>[6x]MSDEPIIYINGDYLPLSQARVS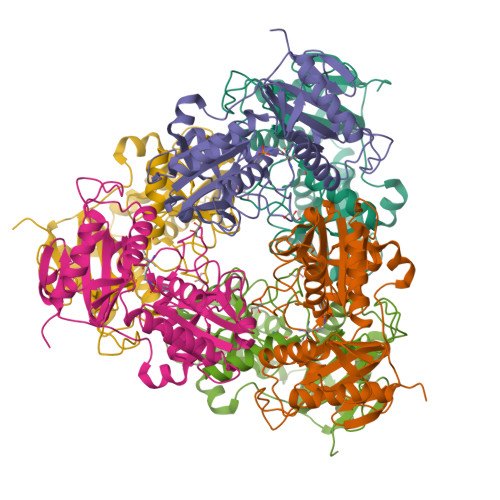PVDQGFLLGDGVFDVVSAWKGNIFKLDAHLDRFFDSIQAARLNHDMSRDAWKEAIIETTRRNGLDDASIRFIVTRGEPKGVVADPRDFKPTCIVWVAPYIFLADEEKRRNGIRLMISATRGFPADTLDPRYKCLDRLHSQLIRLEALEAGYDDALWLDHSGHVSESAASNLFIVKNGVLYTPSAGILRGITRDTILELATELDIPWKERQLSAFDVYIADEVFTCSTAGGALPVREVAGRTIRGTTPGPITQAIDNAYWAMRETDRYATPLSGSHHHHHH>[2x]ATELDVDGVKVRFTNPDKVYFPKLGKNGTKGKLVEYYLSVASGPMLALLRDRPVHLQRFPDGIEGEEIYQKRVPQKHPDYLETCVVTFPSGRTADALKITHPSSIIWAAQMGTVTLHPWQVRCPDTEHPDELRVDLDPQPGTGFKEARTV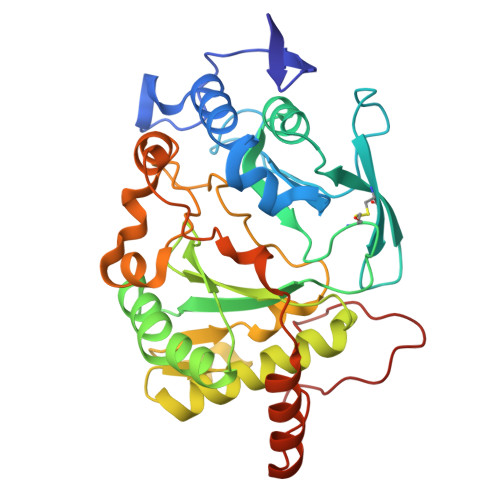ACDVLKPLLDELGLVGYPKTSGGRGVHVFLRIKPQWDFIEVRRAGIALAREVERRAPDAVTTSWWKEERGERLFIDYNQNARDRTFASAYSVRKTPIATVSMPLSWDELRNADPDDYTMNTVPDLLAGRDDPWADIDSVQQSLGPLLDLVAADEERGLGDLPYPPNYPKMPGEPPRVQPSK> MSQSNRELVVDFLSYKLSQKGYSWSQFSDVEENRTEAPEETEAERETPSAINGNP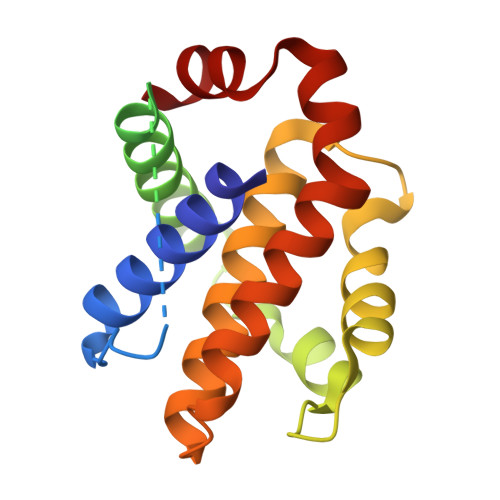SWHLADSPAVNGATGHSSSLDAREVIPMAAVKQALREAGDEFELRYRRAFSDLTSQLHITPGTAYQSFEQVVNELFRDGVNWGRIVAFFSFGGALCVESVDKEMQVLVSRIASWMATYLNDHLEPWIQENGGWDTFVDLYG The first structural representative of the domain of unknown function DUF2006 family, also known as Pfam family PF09410, comprises a lipocalin-like fold with domain duplication. The NE1406 gene of Nitrosomonas europaea, an obligate chemolithoautotroph, encodes a protein with a molecular weight of 40.1 kDa (residues 1–356) and a calculated isoelectric point of 5.0. NE1406 adopts a lipocalin-like fold with domain duplication. The finding of the calycin signature in the N-­terminal domain, combined with remote sequence similarity to two other protein families (PF07143 and PF08622) implicated in isoprenoid metabolism and the oxidative stress response, support an involvement in lipid metabolism.

The final model includes 643 residues in two protein molecules (A and B), two CHES molecules, three glycerol molecules, one sulfate ion and 394 water molecules in the asymmetric unit. The two chains are nearly identical, with an r.m.s.d. of 0.30 Å over 320 Cα atoms (0.60 Å over all 2524 equivalent atoms). The C-terminal domain (residues 221–352) is arranged perpendicular to the long axis of the N-terminal barrel and comprises ten β-strands. In the NE1406 crystal structure, the two lipocalin-like barrels lack the large internal cavity that is typical of lipocalins and also the long structurally flexible loops at the open end of the β-barrel. In fact, only one of the β-­barrel domains of NE1406 harbors a small glycerol molecule from the crystallization solution as a ligand. However, the complete internalization of the glycerol molecule in the NE1406 structure suggests that the N-terminal lipocalin-like barrel might adopt different conformations in the presence of a natural ligand. We therefore propose that this region, which encompasses the calycin signature, acts as a ligand-binding site, the shape and accessibility of which may change with natural ligands. The two barrels are stabilized in a perpendicular orientation with respect to each other. The mainly aromatic and hydrophobic residues implicated in the interaction with CHES are highly or strictly conserved among DUF2006 homologs, suggesting that the domain interface plays a functional role. As with the glycerol molecule bound within the N-terminal barrel, the CHES molecule is also fully enclosed within NE1406 with no exposure to solvent, suggesting some flexibility at the interdomain interface to accommodate ligands.

>GVLAPVVPGKALEFPQDFGAHNDFRIEWWYVTGWLETPTGKPLGFQITFFRTATEIDRDNPSHFAPDQLIIAHVALSDPAIGKLQHDQKIARAGFDLAYARTGNTDVKLDDWIFVRETDGRYRTRIEAEDFTLTFILTPSQPLMLQGENGFSRKGPGAPQASYYYSEPHLQVSGIINRQGEDIPVTGTAWLDREWSSEYLDPNAAGWDWISANLDDGSALMAFQIRGKDDSKIWAYAALRDASGHTRLFTPDQVSFHPIRTWRSARTQAVYPVATRVLTGETEWQITPLMDDQELDSRASAGAVYWEGAVTFTRDGQPAGRGYMELTGYVRPLSM[2x]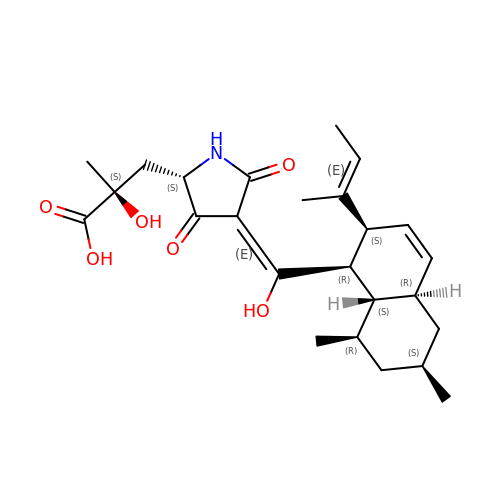(2S)-3-[(2S,4E)-4-[[(1R,2S,4aR,6S,8R,8aS)-2-[(E)-but-2-en-2-yl]-6,8-dimethyl-1,2,4a,5,6,7,8,8a-octahydronaphthalen-1-yl]-oxidanyl-methylidene]-3,5-bis(oxidanylidene)pyrrolidin-2-yl]-2-methyl-2-oxidanyl-propanoic acid | C25 H35 N O6 | AVZATKWNGXCSDN-RQCLIRHHSA-N>[2x]MKIVVITEKPFAENAVKGIREILEKAGHEVVMIEKYKKKEDVIERIKDADGVIVRSDKIDEEIIKAGEKVKIIVRAGAGYDNIDIEACNQGKIVVMNTPGQNRNGVAELCIGMMIFGFRKGFKEGKGRELKDKTLGICGCGYVGKRVKEIAEGIGMKIKVYDPFITTENQVKKIEELFEECQVISLHLPLTKETKGKIGYELIKKLPYGGMICNTARKEIIDEEGLIRIMREREDLIYITDVAPTSKV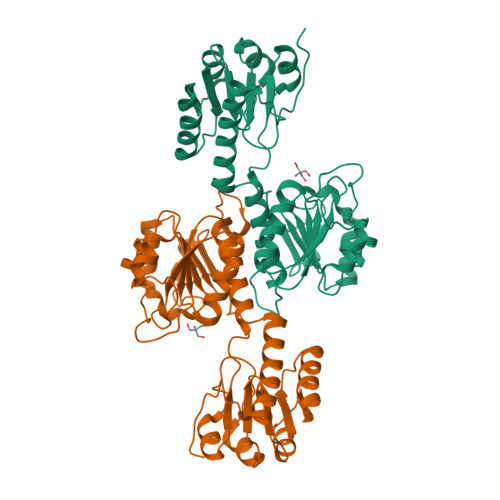FNNEFKGRFFATPIKIGAETEESNINAGMAAASQICDFFTNGTVKFQVNKFLEHHHHHH(1S,3R,5Z,7E,20S,23S)-1,3-dihydroxy-23,26-epoxy-9,10-secocholesta-5,7,10,25(27)-tetraen-26-one 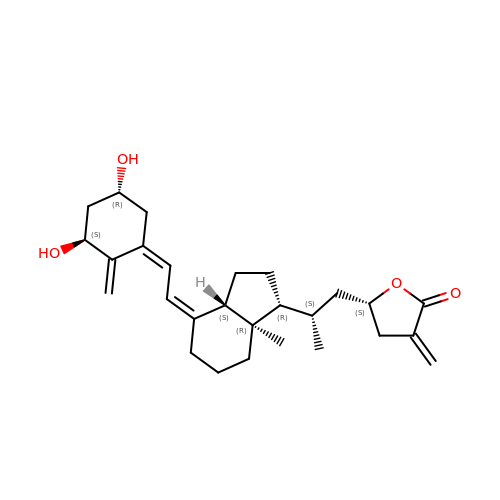| C27 H38 O4 | SAODSJHDCZTVAT-HPNZEMCUSA-N>MISSQQAMVHVVSRNAEGVIVVDGKAYPMAEELVATESVIQRSIKAVAKQIADFYRPLSHRDTHGGGGVAPISDENPLIIISVLKGSYIFTADMVRYLGDYGLPHVVDFLRVASYRGTSSTNKMQLLAETQFKALRGKHVLILEDIVDSGKTLRY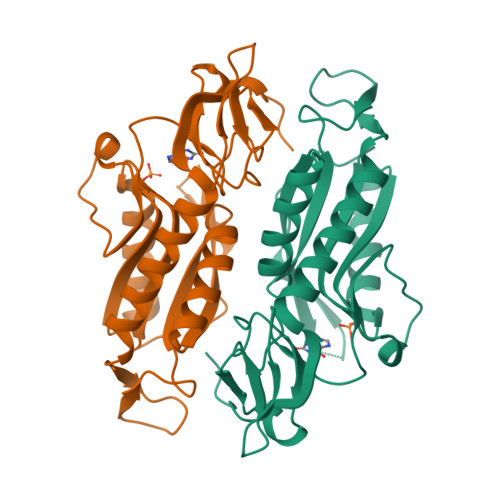ILDKVQREHQPATLKVCVLADKPGGRRVTMQPDFVCLTVPNKYVIGYGFEVNDRFRCFRHIFTLRPGEARRYPAHL[2x]>ALLQKTRIINSMLQAAAGKPVNFKEMAETLRDVIDSNIFVVSRRGKLLGYSINQQIENDRMKKMLEDRQFPEEYTKNLFNVPETSSNLDINSEYTAFPVENRDLFQAGLTTIVPIIGGGERLGTLILSRLQDQFNDDDLILAEYGATVVGMEILREKAEEIEEEARSKAVVQMAISSLSYSELEAIEHIFEELDGNEGLLVASKIADRVGITRSVIVNALRKLESAGVIESRSLGMKGTYIKVLNNKFLIELENLKSHHHHHH[2x]

In low G + C Gram-positive bacteria, CodY is a global regulatory protein that controls the transcription of numerous genes. CodY from B. subtilis and most other low G + C Gram-positive bacteria is a DNA-binding protein that is activated by the branched-chain amino acids (BCAAs),2 leucine, isoleucine and valine, which may be viewed as signals of the metabolic status of the cell, and GTP, which may signal the energetic status of the cell. CodY from B. subtilis consists of 259 amino acid residues. The structures of full-length CodY from B. subtilis determined here reveal the effector binding domain and the DNA binding domain as discrete entities separated by a helical linker.

We have solved the structure of unliganded CodY in three different crystal forms containing 14 (form A), 10 (form B), and 2 (form C) molecules in the asymmetric unit from data sets extending to 4.6, 3.0, and 3.7 Å spacing, respectively. Examination of the molecular packing in the crystals of unliganded CodY reveals that the basic building block of all three crystals is a tetramer. The tetramer in the form C crystals and one of the tetramers in both the form A and the form B crystals are generated by crystallographic 2-fold symmetry. Superposition of the eight tetramers from the three crystal forms suggests that they are essentially identical within the limits of the data. In the crystals, four CodY protomers are assembled into an unusual tetramer in which four wHTH domains are sandwiched between two GAF domain dimers. For the unliganded form in particular, the tetramer is compact with extensive subunit interfaces. From within this tetramer structure, there is no possibility that the wHTH domains of CodY could bind to DNA in a conventional manner, because the GAF domains of partner subunits in the tetramer occupy a substantial volume that would be taken up by the DNA duplex.>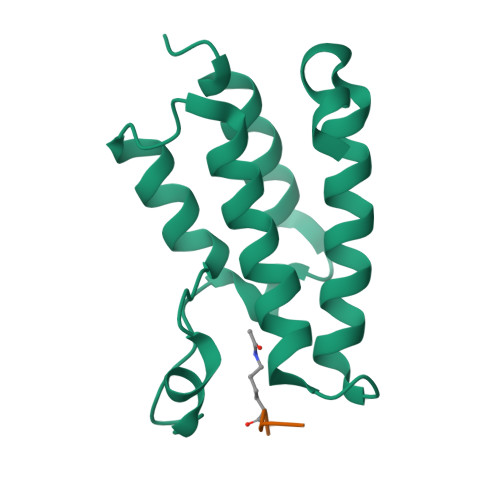 AMANIAQRPKRGPHDAAIQNILTELQNHAAAWPFLQPVNKEEVPDYYDFIKEPMDLSTMEIKLESNKYQKMEDFIYDARLVFNNCRMYNGENTSYYKYANRLEKFFNNKVKEIPEYSHLID;> AKRHRKILRNSIQGI>MASTDYHVDLTNCDREPIHIPGYIQPHGCLIACDNAMRMVLRHSENCGELLGLEGDLNGRTAEDVLGKRLVHDLRNALTVTGKTTRPAMLPAMETSDGRSFDISLHRYKSTTIIEFEPSDSDTQPLGTARKMVDRIREADSVESLISRTTRLVKATLGYDRVLIYRFEEDGAGKVVSEAKQPELESFLGQYFPASDIPQQARALYLKNTLRIISDASGTPIPVLPAVDVSGEPLDLSYAHLRNFSPIHCEYLRNMGVAASM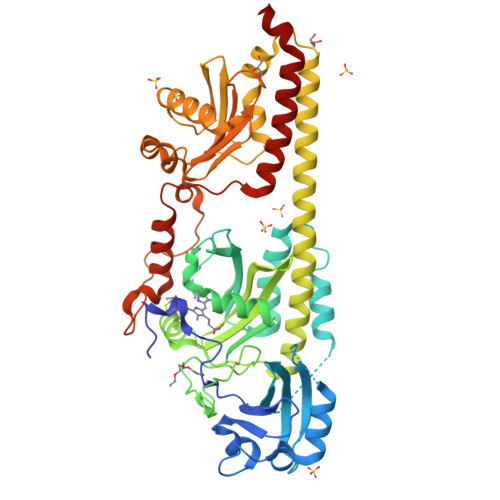SISVIVDDALWGLIVCHHCSPRVLSMPVRIAAAMFGEFFSMFLQVLKQKRRLDTINHAHAALDRFLRLAAHRANLEELLVDSFQDFARLIPCDGVGLWVGNNWHGHGATPPHDAIPRLARFVASVSEGRVWATHALSQAIPEAEIYADTAAGMLAIPISQVKSDYLLFFRKEIVQNLNWAGNPEKSYETGPMGDRLTPRKSFAIWKESVRLQAQPWSEADREIAETARIALVGVAFHHSELMAGLEYK[2x]> MEGMVFSLKYLGMTLVERPKGEELSAAAVKRIVATAKASGKKLQKVTLKVSPRGIILTDSLTSQLIENVSIYRISYCTADKMHDKVFAYIAQSQQNESLECHAFLCTKRKVAQAVTLTVAQAFK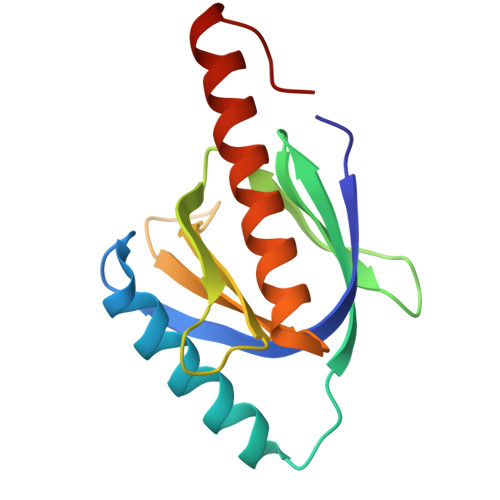VAFEFWQVSLVPR>[8x]MKADAVKIADGVYWVGVLDWDIRMYHGYTLNGTTY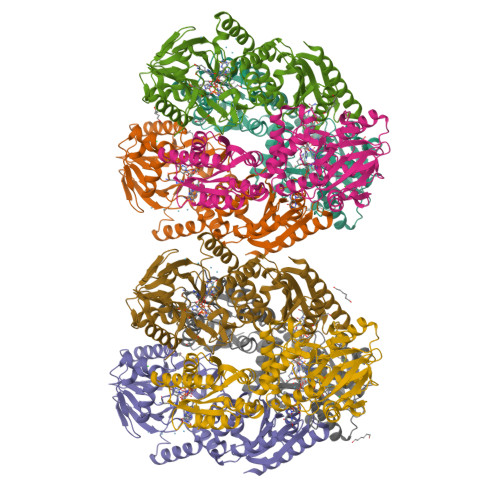NAYLVFGDDKVALIDNTYPGTSAQMWGRIKDACEKEGREFKIDVIVQNHVEKDHSGALPEIHKKFPEAPIYCTEVAVEGLVKHFPSLKGAPFKVVKSLESIDLGGKTLTFLEAPLLHWPDSMFTLYAEEGILFSNDAFGQHLCFTQRFDHEIPENILMDANQKFYANLITPLSKLVLKKFKEVIELGLLEKIKMIAPSHGQIWTDPMKVIGAYQDFATGKCKDKVTIVYDTMHGSTQKMAHAFAEGIMSEGVDVKMYFLHNDERSEIVKDILDSKAFLLGAPTIYDEPFPSVGDLIYYLKGLKFNRTGLKRLALAFGSMGGNGGGTKVLAEKLKECGFEVLDEYELYYVPTEDELEKCYNMGKRLAVKVKEMKTE> MDKEE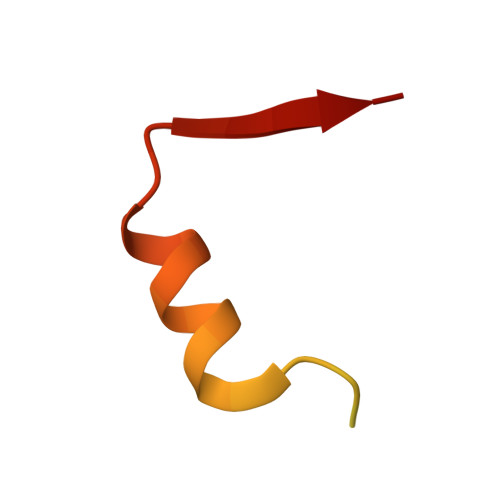VKREMKEQEGNPEVKSKRREVHMEILSEQVKSDIENSRLIVAN>[11x]MSYHKENTPLTAGSQAASSSTASYQTPPYAPPSSVNHQQQQQARAAAPSYVGPTPTSTTTYPTIFTPGGFGAPPPSDPEAEEKYIERQLKYLGPISQVSDAYRLDTTTLKIEFDDSFPEVSKPGPALESVRKLNRILYEGMSDAIHIIFSLFLGFLAAITVGFFMGMARFMYTYMAGPFNQLMFLLIASLAPSWRAFFRAGMDPIFESGSLALSNIQVRLGMEGKARHKELKD

Caveolins are a unique family of membrane remodeling proteins present broadly across animals (Metazoa), and in vertebrates form flask-shaped invaginations known as caveolae. Unlike vesicle coat proteins such as clathrin, COPI, and COPII that cycle on and off membranes and share evolutionary origins and structural features, caveolins are unrelated in sequence to other vesicle coat proteins and remain integrated in membranes throughout their life cycle. Using a combination of computational and structural approaches, we now show that caveolins across evolution share the ability to assemble into amphipathic disk–shaped multimers composed of spiraling α-helices and a central protruding parallel β-barrel. Each complex forms a disk with 11 spiraling α-helices and a central β-barrel, with each protomer forming contacts with two protomers to the left and two to the right.

We next determined a 2.9 Å resolution cryo-EM structure of the S. rosetta caveolin complex. A model of S. rosetta caveolin spanning amino acids 79–231 was built from the density map. The S. rosetta caveolin complex, ∼127 Å in diameter and ∼46 Å in height, is a disk composed of spiraling α-helices with a central β-barrel. The variable N-terminal region forms a short α-helix that is positioned about halfway up the β-barrel before snaking along the cytoplasmic-facing surface of the complex. Each protomer makes a 180° turn at the hook structure, which is followed by the spoke region. The α-1 helix forms the rim at the edge of the disk that is ∼16 Å in height. Finally, S. rosetta caveolin has a C-terminal β-strand that forms a parallel β-barrel with a diameter of ∼30 Å and contributes to the ∼46 Å overall height of the complex. The detergent micelle surrounds the hydrophobic face of the disk and reaches into the β-barrel. As a result, in the S. rosetta complex, additional contacts are made with the i + 5 and i − 5 protomers as the variable N-terminal region of i rises up the central β-barrel and contacts the C-terminal β strands of i + 5 and i − 5. The three β-barrels have a similar outer diameter of ∼28–30 Å; however, the S. rosetta caveolin complex’s central β-barrel is ∼10 Å longer than the other caveolin complexes.>XAXAEAAEKAAKY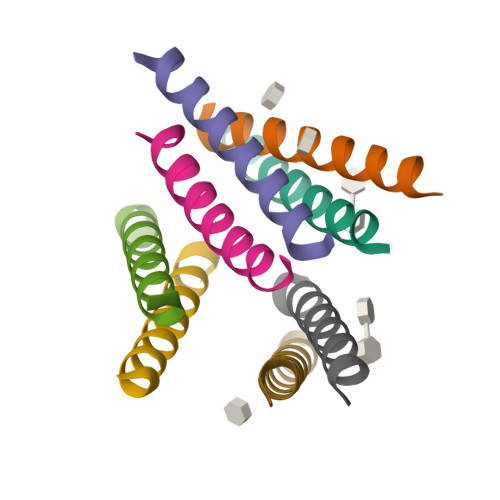AAEAAEKAAKAXAX[12x]>GSMAKVQVNNVVVLDNPSPFYNPFQFEITFECIEDLSEDLEWKIIYVGS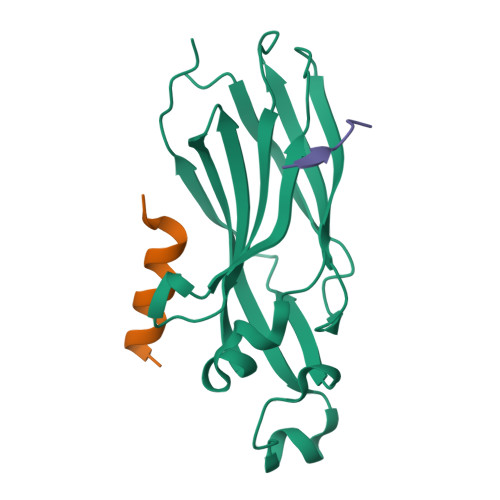AESEEYDQVLDSVLVGPVPAGRHMFVFQADAPNPGLIPDADAVGVTVVLITCTYRGQEFIRVGYYVNNEYTETELRENPPVKPDFSKLQRNILASNPRVTRFHINWED[8x];>EELHSLDPRRQELLEARFTGV[16x]> GTKFSKEQLRTFQMIHENFGRALSTYLSGRLRTFVDVEISIDQLTYEEFIRSVMIPSFIVIFTGDVFEGSAIFEMRLDLFYTMLDIIMGGPGENPPNRPPTEIETSIM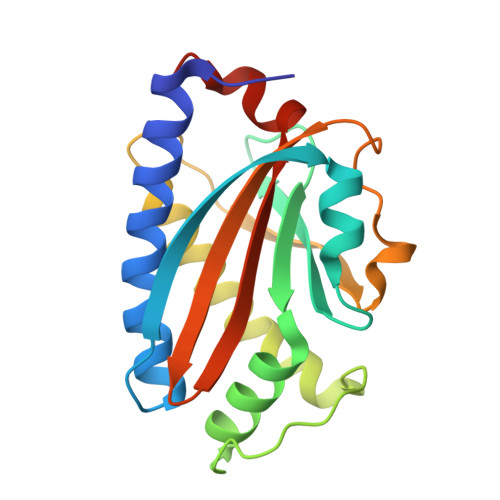RKEVTNMLTLLAQAWSDFQYFIPSIENVETNPQFVQIVPPNEIVLLVTASVSWGEFTSFINVCWPFSLLEPLLEKLSDR(4S,7R)-7-hydroxy-1-(4-methoxybenzyl)-7-methyl-4,5,6,7-tetrahydro-1H-benzotriazol-4-yl 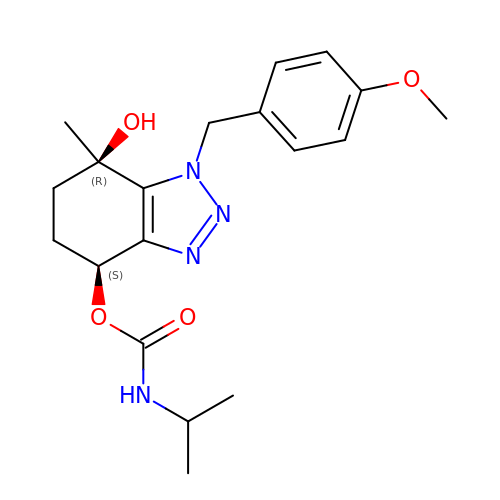propan-2-ylcarbamate | C19 H26 N4 O4 | CDAJJINZTVFCPA-HNAYVOBHSA-N> MPKALRFLGWPVLVGVLLALLIIQHNPELVGLPRQEVHVEQAPLLSRLQEGPVSYANAVSRAAPAVANLYTTKMVSKPSHPLFDDPMFRRFFGDNLPQQKRMESSLGSAVIMSAEGYLLTNNHVTAGADQIIVALRDGRETIAQLVGSDPETDLAVLKIDLKNLPAMTLGRSDGIRTGDVCLAIGNPFGVGQTVTMGIISA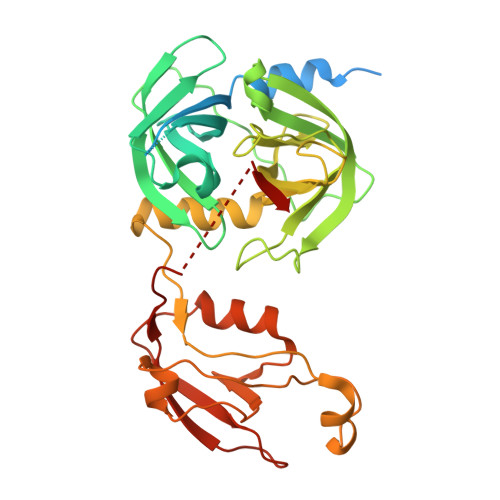TGRNQLGLNTYEDFIQTDAAINPGNAGGALVDAAGNLIGINTAIFSKSGGSQGIGFAIPTKLALEVMQSIIEHGQVIRGWLGVEVKALTPELAESLGLGETAGIVVAGVYRDGPAARGGLLPGDVILTIDKQEASDGRRSMNQVARTRPGQKISIVVLRNGQKVNLTAEVGLRPPPAPAPQQKQDGGE> GNCWLRQAKNGRCQVLYKTELSKEECCSTGRLSTSWTEEDVNDNTLFKWMIFNGGAPNCIPCKETCENVDCGPGKKCRMNKKNKPRCVCAPDCSNITWKGPVCGLDGKTYRNECALLKARCKEQPELEVQYQGRCKKTCRDVFCPGSSTCVVDQTNNAYCVTCNRICPEPASSEQYLCGNDGVTYSSACHLRKATCLLGRSIGLAYEGKCIKAKSCEDIQCTGGKKCLWDFKVGR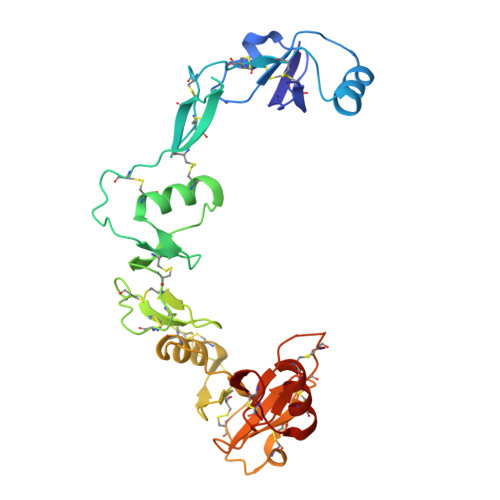GRCSLCDELCPDSKSDEPVCASDNATYASECAMKEAACSSGVLLEVKHSGSCN(2'S,3R,4'S,5'R)-N-(2-aminoethyl)-6-chloro-4'-(3-chloro-2-fluorophenyl)-2'-(2,2-dimethylpropyl)-2-oxo-1,2-dihydrospiro[indole-3,3'-pyrrolidine]-5'-carboxamide 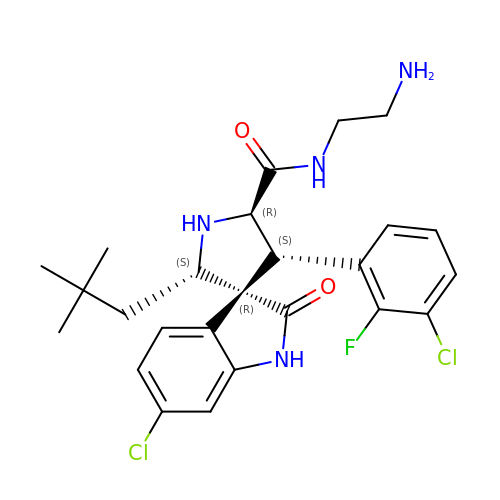| C25 H29 Cl2 F N4 O2 | FNYZLFJBIYJBIK-MZFHRINRSA-N> VRPLNCIVAVSQNMGIGKNGDLPWPPLRNEFKYFQRMTTTSSVEGKQNLVIMGRKTWFSIPEKNRPLKDRINIVLSRELKEPPRGAHFLAKSLDDALR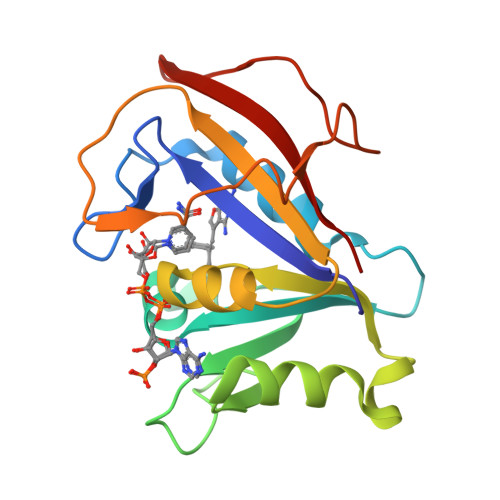LIEQPDLASKVDMVWIVGGSSVYQEAMNQPGHLRLFVTRIMQEFESDTFFPEIDLGKYKLLPEYPGVLSEVQEEKGIKYKFEVYEKKD>[4x]MAHHHHHHMSAPSKPSDAVARGTLYIVAAPSGAGKSSIVNATLARDPQIALSISFTSRAMRPGEVNGQHYHFVSAEKFEQMIAAGDFF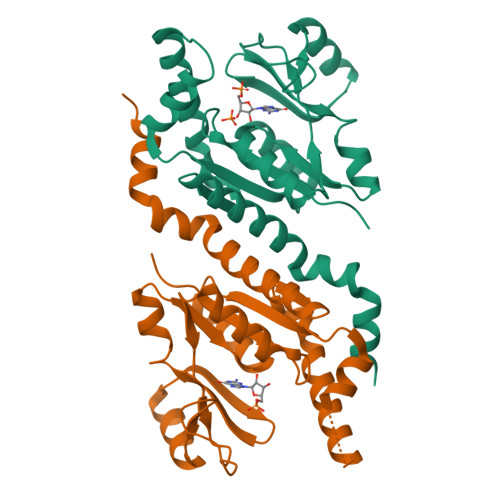EHAWVHGDWKGTARQSVEPQLAAGQDVLLEIDWQGAQQVRQLVPGTVTVFILPPSKQALQDRMRKRGQDSEAVIAQRLGAARDEMLHFNEFDYVIVNEVFDTAVDELCAIFTASRLRREAQKVRHAGLIQALLTPDPGATD>[2x]GMS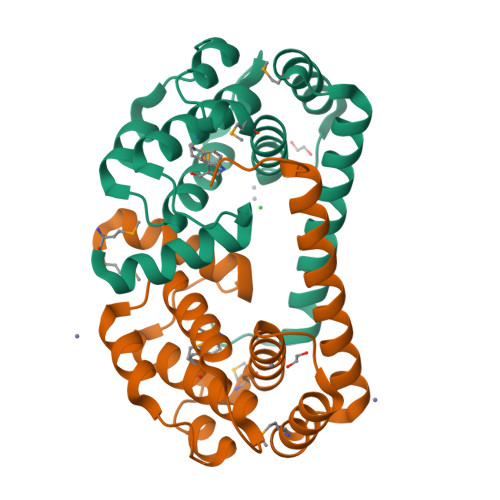DIKKLGSSWIINWFFGFNQIPTNEDSSIYMKSVLTCAKADGVISPEEKDWALGFCASWGVADWVIEDLKTYEADEALEEVIARSPQVSMAQRDILLSAIWVSAADGELHEKEKAKIRKMATILGIKEEIVDQLEQLYYYEAALRQKRLNLLYPQKSPY>AKLETVTLGNIGKDGKQTLVLNPRGVNPTNGVASLSQKGAVPALEKRVTVSVSQPSRNRKNYKVQVKIQNPTACTANGS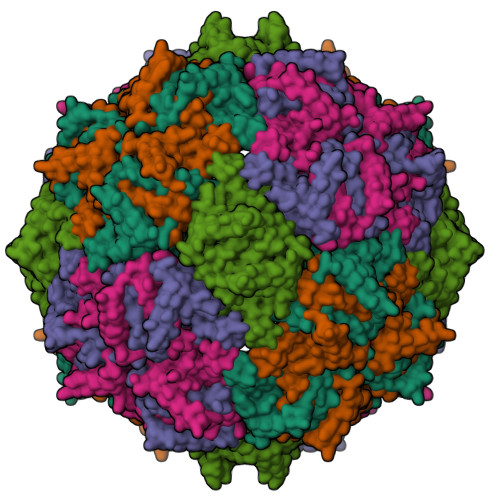CDPSVTRQAYADVTFSFTQYSTDEERAFVRTELAALLASPLLIDAIDQLNPAY[5x]O-(2-aminoethyl)-L-serine | C5 H12 N2 O3 | 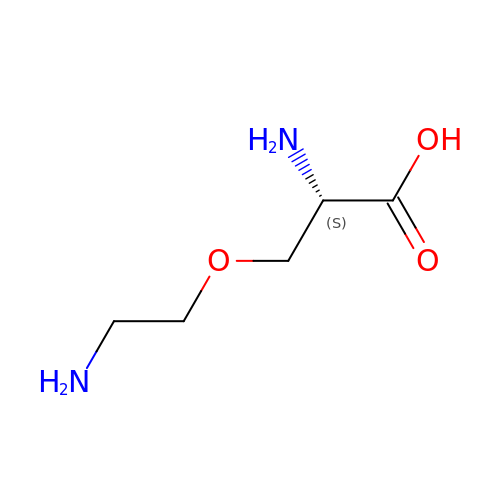SLTGLTLBIVDQKE-BYPYZUCNSA-N>[2x]AHPWHDLEIGPGAPQIFNVVVEITKGSKVKYELDKKTGLIK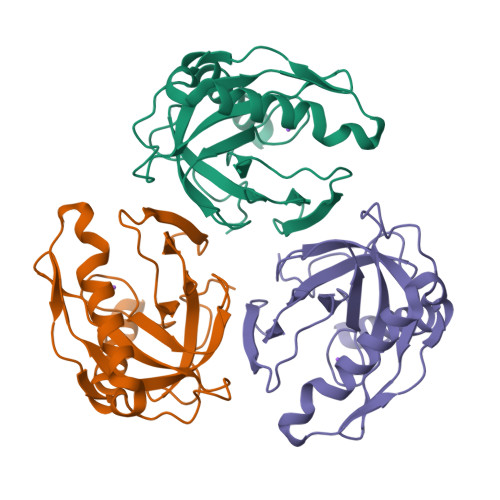VDRILYSSVVYPHNYGFVPRTLCEDNDPIDVLVIMQEPVLPGCFLRARAIGLMPMIDQGEKDDKIIAVCVDDPEYKHYTDIKELPPHRLSEIRRFFEDYKKNENKEVAVNDFLPSESAVEAIQYSMDLYAEYILHTLRR> ETGQTLAANIWSDKTTAQNEPINLTNANAPIKNAKNLNSTITNVAAFDTKLNHLLVDTITGRVFVGGVNRLYQLSPDLELSE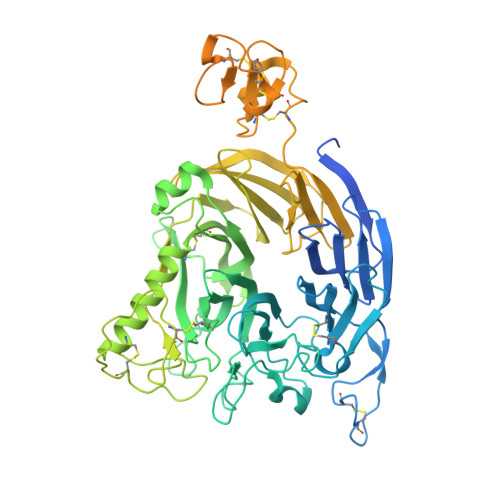TVKTGPQNDSVECSILDCPLNAVRSPTDNYNKVLLIDRATSRLIACGSLFQGTCTVRNLQNVSIIEHEVPDAVVANDANSSTVAFIAPGPPQHPVTNVMYVGVTYTNNSPYRSEIPAVASRSLEKTKMFQIASSAVTTGTRTFINSYARETYFVNYVYGFSSERFSYFLTTQLKHSHHSSPKEYITKLVRICQEDSNYYSYTEIPVECISDAQGGTKFNLVQAGFLGKPSSDLAQSLGISIQDDVLFAVFSKGEGNTPTNNSALCIYSLKSIRRKFMQNIKSCFNGSGMRGLDFISPSMPCVLTKLQTIGEDFCGLDVNSPLGGETPITSVPVAMFNTKLTSVAATSTSGYTVVFVGTSDGFLKKVVIESSSIANEYASFAVDLGSEINRDMQFDNQNLYIYVMSKTKVSKVKVFDCSDYKTCGDCLGARDPYCGWCSLENKCSPRSNCQDDANDPLYWVSYKTGKCTTITSVVPHQLQRTTARTLELIIDHLPQLKENLICAFTTEDKALFTNATKKRNGVNCTTPRTDMLPQIEQGKHHFTAKLSVRTRNGPDLVSTDFTFFDCSTHSSCTRCVSSEFPCDWCVEAHRCTHDTAENCRNDILVTGVSRIGPSYRSGPGFCPTGTKHHHHHH>[2x]MQEKSKMDCHGGI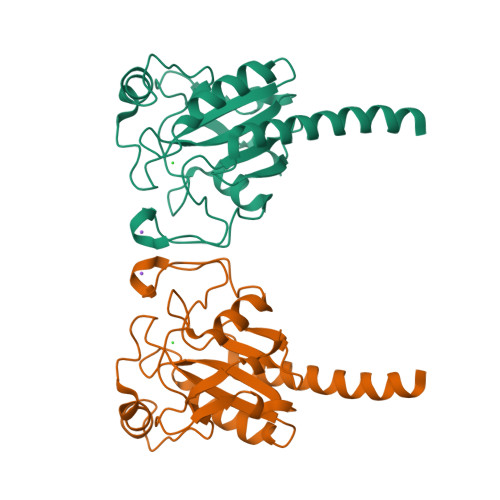SGTIYEYGALTIDGEEYIPFKQYAGKYVLFVNVASYGGLTGQYIELNALQEELAPFGLVILGFPCNQFGKQEPGENSEILPTLKYVRPGGGFVPNFQLFEKGDVNGEKEQKFYTFLKNSCPPTSELLGTSDRLFWEPMKVHDIRWNFEKFLVGPDGIPIMRWHHRTTVSNVKMDILSYMRRQAALGVAENLYFQ>MAAGESMAQRMVWVDLEMTGLDIEKDQIIEMACLITDSDLNILAEGPNLIIKQPDELLDSMSDWCKEHHGKSGLTKAVKESTITLQQAEYEFLSFVRQQTPPGLCPLAGNSVHEDKKFLDKYMPQFMKHLHYRIIDVSTVKELCRRWYPEEYEFAPKKAASHRALDDISESI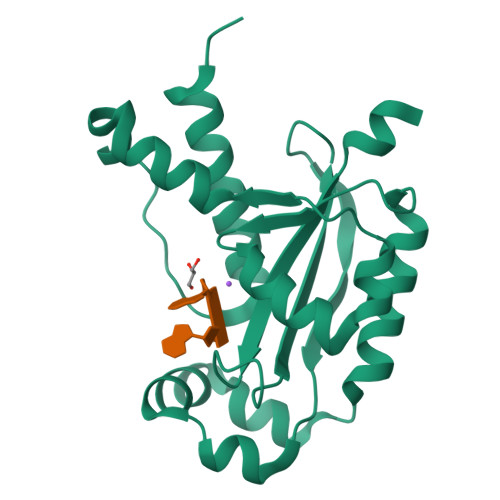KELQFYRNNIFKKKIDEKKRKIIENGENEKTVS[2x]N-phenyl-N'-pyridin-3-ylurea 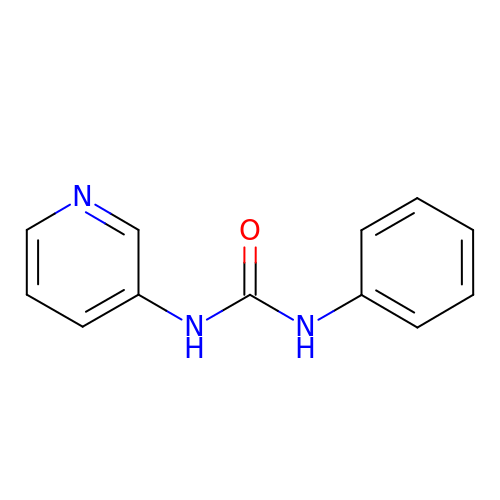| C12 H11 N3 O | WBKYYDBHEGTTON-UHFFFAOYSA-N> SPNVEACGYSDRVQQITLGNSTITTQEAANAVVCYAEWPEYLPDVDASDVNKTSKPDTSVCRFYTLDSKTWTTGSKGWCWKLPDALKDMGVFGQNMFFHSLGRSGYTVHVQCNATKFHSGCLLVVVIPEHQLASHEGGNVSVKYTFTHPGERGIDLSSANEVGGPVKDVIYNMNGTLLGNLLIFPHQFINLRTNNTATIVIPYINSVPIDSMTRH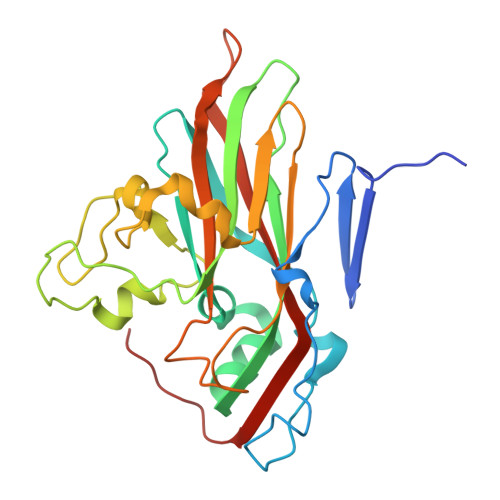NNVSLMVIPIAPLTVPTGATPSLPITVTIAPMCTEFSGIRSKSIVPQ1,3-DIAMINOPROPANE | 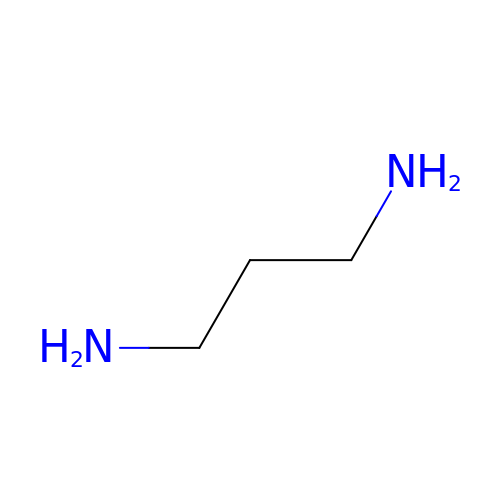C3 H10 N2 | XFNJVJPLKCPIBV-UHFFFAOYSA-N>SMITKYLYDENAYDYHDGGYRPLKKAPGEEHPLNVPAFLKPDRIEGNEIYYTVTAQAGETKILPGKPTHTWGYNGSILGPAIQFETGKTYHVTLKNELDEVTTFHWHGLNIVGPYEDGGPHAPVYPHGERKITFTVDQPAANIWLHPHPCPETARQVWNGLAAPVIITDGHEQSLKLPRRWGVNDFPVVLQDRSYHDNQLDYKADYDVDGTLGDYALVNGTVNPVVNVTKPIVRLRFLNGSNRREWRLHFADYHPFTQIGSDGGLLPEAVKMDRIMLTCAERADVLVNFSDYQPGQEVILQTDDFDLIKFKIGDIKKENMLLPSPLAEIPALSVDENTPVFKTVMSGMDDQVRLDGKLFDMQRIDTRQQVDQTQIWEVSNTNDMEGGMIHPFHIHGCQFQLIDRNGHAVNPNEHGWKDTIGVNPNETVRIKV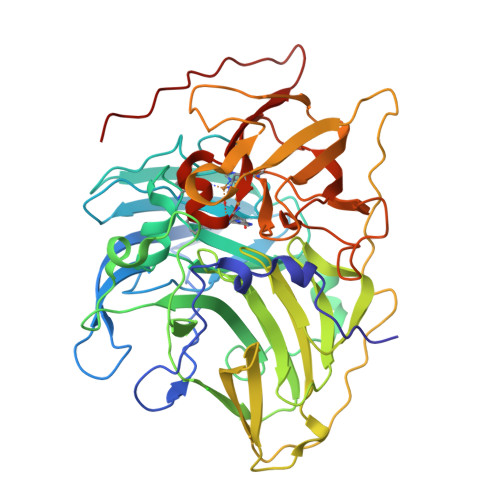KFTKLGIFMYHCHILEHEDTGMMAQIEIFDPDHPIEYHLMPMNHK[2x]> MRAVIQRVKKSWVEVDGKVVGSINEGLNVFLGVRKGDTEEDIEKLVNKILNLRIFEDERGKFQYSVLDIKGEILVVSQFTLYANVKKGRRPSFEEAEEPKR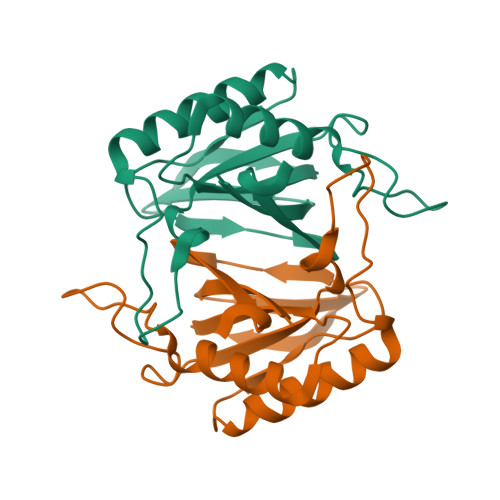AKELYEKFVDKIKESGLKVETGIFGAMMDVFIENWGPVTIIIDSREI>[4x]MTRRILVTGSSRGIGKAIALQLAKAGFDVTVHARSRQAEAEQVVQEIQALGQNSHYLMFDVNERQTVQQILEQDVEQHGGFYGVVLNAGLTHDGAFP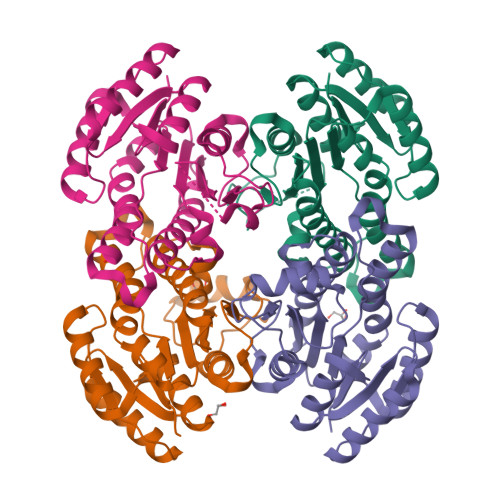ALTDQDWDEVISTSLDGFYNVLKPLIMPMIHLRKGGRIVTLSSVSGIMGNRGQVNYSAAKAGLIGATKALALELAKRKITVNCVAPGLIETEMVTDEVKEHALKMIPLQRMGQVDEVASVVKFLCSDEASYVTRQVISVNGGLI The enzyme, encoded by the pabC gene, is labeled as PabC. Chorismate is first converted to 2-amino-2-deoxyisochorismate before production of 4-amino-4-deoxychorismate, which is then converted to PABA and pyruvate by PabC. PABA is required for the biosynthesis of folic acid and by extension also of essential metabolites such as thymidylate and methionine. The absence of the enzyme in humans and its essentiality in various microbes suggests that inhibition of PabC offers the possibility of new therapies targeting a range of microbial infections and structural studies provide useful data to assess the potential of this protein for such early stage drug discovery.

We describe the construction of an efficient bacterial recombinant expression system, enzyme purification and crystallization protocols, and report the high-resolution crystal structure of PabC from P. aeruginosa (PaPabC). In the crystal structure two polypeptide chains, labelled A and chain B together constitute the asymmetric unit in PaPabC, and the crystals have an estimated bulk solvent content of 45%. The polypeptide chains form a dimer and such oligomerization is required to create the enzyme active site. The PaPabC subunit is constructed from two domains. The active site is formed in a cleft formed between the two domains. The PLP cofactor is covalently bound to Lys140 that is in domain II. The PLP phosphate accepts hydrogen bonds donated by a cluster of main chain amide groups from Val200, Met201 and Ser237, and the side chain of Arg46. Tyr92 from the partner subunit forms a hydrogen bond to PLP O3. Given the importance of such complexes we judged it important to get such data and attempted to determine structures of PaPabC in complex with a number of compounds, for example, the sample used for structure determination was crystallized in the presence of 10 mM PABA. However, we have been unable to identify electron density compatible with binding of any such ligand in the substrate-binding pocket.

>[2x]MGSSHHHHHHSSGENLYFQGHMLDWVDGRPAAELSVRDRGLAYGDGLFETLAVRAGTPRLLERHLARLEEGCRRLAIPLDTAALRQELLAFCAALGDGVAKLIVTRGEGLRGYAPPAEASPRRILSGSPRPAYPERHWQQGVRLFACRTRLAEQPLLAGLKHLNRLEQVLARAEWSDAGHAEGLMLDVHERVVEGVFSNLLLVLDGTLVAPDLRRCGVAGVMRAELLERAEGIGVPLAIRDVSMAELATADEVFLCNSQFGIWPVRALDEHVWPVGELTRKLQDQLRDDLDF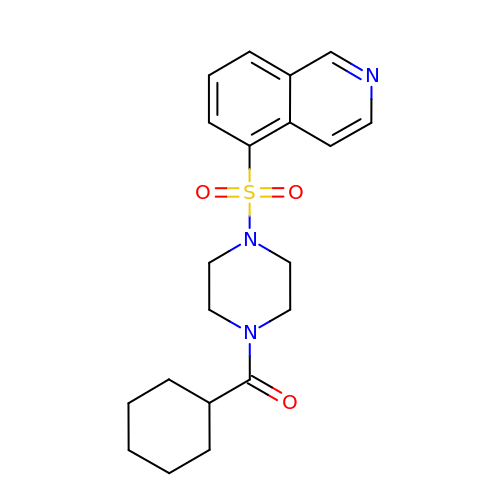cyclohexyl{4-[(isoquinolin-5-yl)sulfonyl]piperazin-1-yl}methanone | C20 H25 N3 O3 S | RQGSIJUNMAAIRB-UHFFFAOYSA-N> MRGSHHHHHHGRSLNPLSTPQFDSTDETPASYNLAVRRAAPAVVNVYNRGLNTNSHNQLEIRTLGSGVIMDQRGYIITNKHVINDADQIIVALQDGRVFEALLVGSDSLTDLAVLKINATGGLPTIPINARRVPHIGDVVLAIGNPYNLGQTITQGIISATGRIGLNPTGR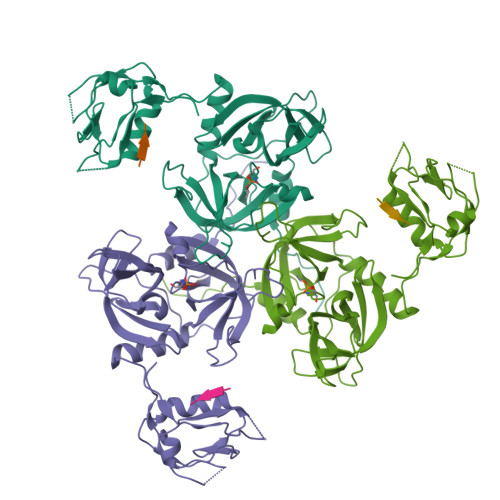QNFLQTDASINPGNSGGALVNSLGELMGINTLSFDKSNDGETPEGIGFAIPFQLATKIMDKLIRDGRVIRGYIGIGGREIAPLHAQGGGIDQLQGIVVNEVSPDGPAANAGIQVNDLIISVDNKPAISALETMAQVAEIRPGSVIPVVVMRDDKQLTLQVTIQEYPATN;> DNRDGNVYYF> MMAKAKALIPDNGRAGADEGNRQAWIGQEVLRREDRRLLTGTATFAGDLGVPGQLHMRIVRSTQAHARIVSIDATEAEKTPGVRMVITSEHTRHLGSVLLEELGYHEIYENIEDFSHPVLAVDKVLYVGQPVVAVLAVDPYLAEDAAELVSIEYEPLPVLLDPEEALTGK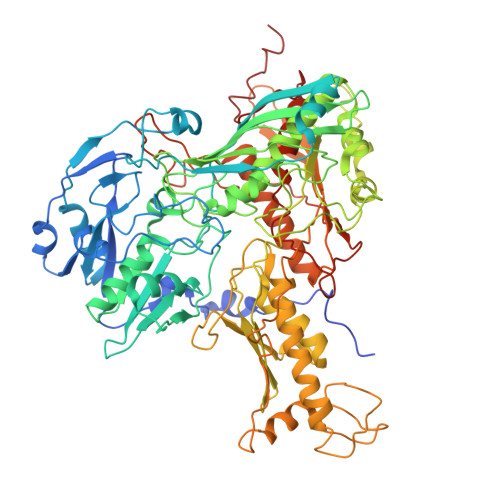VELFPGRGNEGARIKKAYGDIDRAFAEAEHVIRHKYVTNRHSGVPMEPRAVVVQPDPARDTLFIWGTVHVHDNRRIIAKMLNLPEVNVRMKHVEIGGSFGVKGGVFPENVVAAWAARTLGVPIKWTEDRVEHMTSTSHAREMVHKLELALDAEGRILGMKDEIFHNHGAYFRQAEPLVSDITAGIVFGPYRVPAYDATLHAVFTNKTPVGAYRAPGRYESTFARERIFDLACAEIGLSKTEFRRRNLLTAEDLPWTPGLDIVHEPYHFDSGDVVKHFNEALEAANFSEWLEESKRLRADGRKVGVGLGVLMDKAGLGLFETGGVEVSRAGRVTVKTGGSSVGQGIETVLAQIVAEELQIAPENIDIVHSDTELIPDGVGSWSSRSTVLAGGAARKAALAVVEKARRLASEMLEADPDDLELTAGSFKVKGTDQQISLYEIAAARDPFTARADNDEPGLAADAVYMNNAMNYPYGVTLVQIELDPDTGGHRILRFSTSTEAGRVINPLTTRGQIIGAAVQGIGGALYEEFLYEEDGQPITTSFMDYLLPSAQEMPNVDCFVTEDAKSPDNPFGAKGLGEIGIIAAGAAIASAIDDAIADGVHTDRLPVTPEQIFSRCQGLNKAER> EVDKRREINNEHPLLMMPLYANGEEFNQGKYTFWGGDTLTGKWENIPDDLKPYTVIQLHPDDLPKRDGAARDFYEHMLEEAAKYVNPKTGKNEPIPVILTVYTAGNMPYYTSAHWLSTSWIDKMYQKYPNLHGIFSTASYWIWANDIENKAADYLKVSAKNGGYFIWAEQNVGSAIEKAFGKNGKIAFQKSVDKYWKNLIFMFKNTPAAEGNDSTTESYMKGLWLSNHTYQWGGLMDTWKWYETGKWKLFASGNIGKSQGDRQWLTEPESMLGEEALGVYLNGGVVYNFEHPAYTYGVNNKESLLFSEVIKEFFRYVIAHPAPSKEKVLEDTKVFIHGDYSNKGNGKFFVNVNTDREQTPLYMTGRYNVIPAIPGVLKTDKL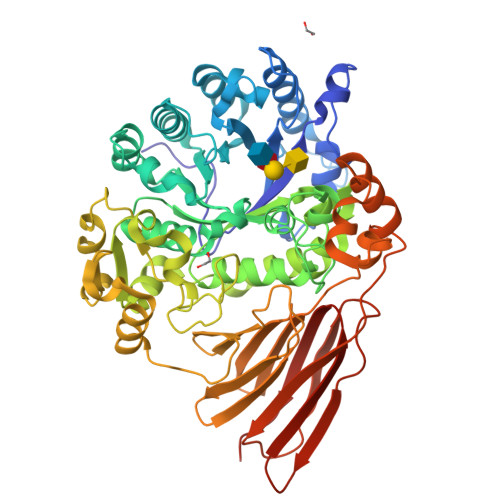KESVSSSRIQIKEITSPEFSSTQARKEYLNKLYPMNYEGDIFAQKLDNRWFVYNYKVNENVKQTGKLKFNSLEMNVEFEPHTYGIFERISNGLKVNLNNFRTNKDSLWSNAQDANQAKKLPQLTKKGAIKWIEEHYIKDTQFGEKRVTKIVLRGIDKLPTIHSLSGTNNSYDQPSLNFDQKNHMVTITINSNGNLEFELHFLEHTRAPPPPPLRSGC> MALTVDVAGPAPWGFRITGGRDFHTPIMVTKVAERGKAKDADLRPGDIIVAINGES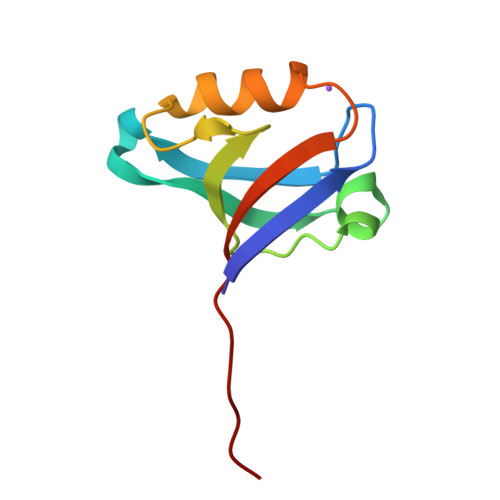AEGMLHAEAQSKIRQSPSPLRLQLDRSTIESEV>MQILWKKYVKENFEMNVDECGIEQGIPGLGYNYEVLKNAVIHYVTKGYGTFKFNGKVYNLKQGDIFILLKGMQVEYVASIDDPWEYYWIGFSGSNANEYLNRTSITNSCVANCEENSKIPQIILNMCEISKTYNPSRSDDILLLKELYSLLYALIEEFPKPFEYKDKELH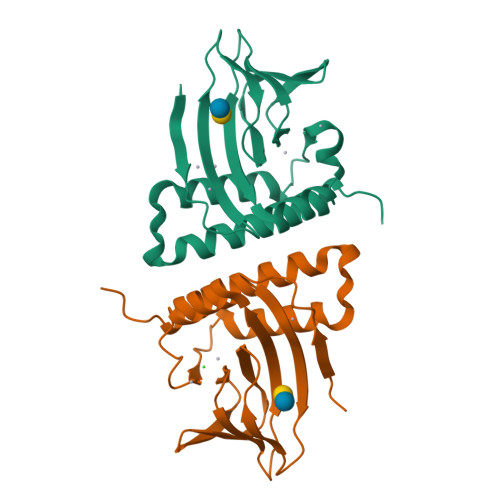LVPRGSHHHHHH[2x]> SMTKDEQFEEYVQNFKRQEAEGTRLQRELRGYLAAIKGMQEASMKLTESLHEVYEPDWYGREDVKMVGEK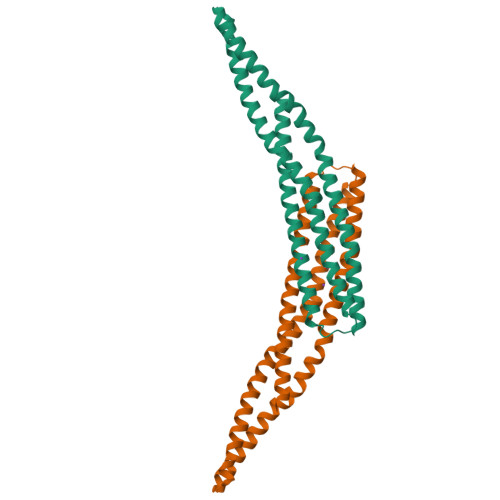CDVLWEDFHQKLVDGSLLTLDTYLGQFPDIKNRIAKRSRKLVDYDSARHHLEALQSSKRKDESRISKAEEEFQKAQKVFEEFNVDLQEELPSLWSRRVGFYVNTFKNVSSLEAKFHKEIAVLCHKLYEVMTKLGD> MVSLFKRGKAPPLTKEGPTSKKPPNTAFRQQRLKAWQPILSPQSVLPLLIFVACIFTPIGIGLIVSATKVQDLTIDYSHCDTKASTTAFEDIPKKYIKYHFKSKVENKPQWRLTENENGEQSCELQFEIPNDIKKSIFIYYKITNFYQNHRRYVQSFDTKQILGEPIKKDDLDTSCSPIRSREDKIIYPCGLIANSMFNDTFSQVLSGIDDTEDYNLTNKHISWSIDRHRFKTTKYNASDIVPPPNWMKKYPDGYTDENLPDIHTWEEFQVWMRTAAFPKFYKLTLKNESASLPKGKYQMNIELNYPISLFGGTKSFVLTTNGAIGGRNMSLGVL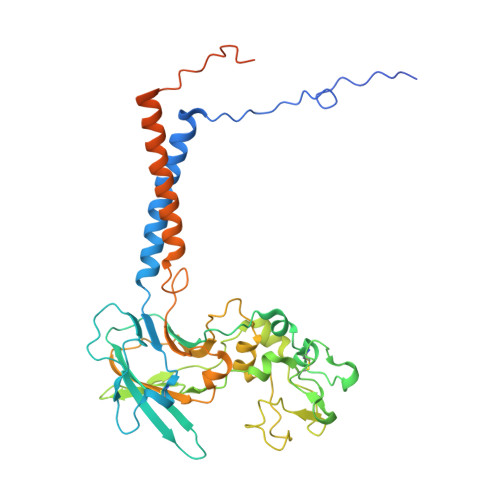YLIVAGLCALFGIIFLVKLIFQPRAMGDHTYLNFDDEENEDYEDVHAENTTLREILGGGGLVPRGSGGHHHHHHHHHH>SYDTVMDKYWLSQYVIARETYDWYTLQKDYETVGMLSSPSEGQSYASQFQGDKALDKQYGSNVRTSVTIVSIVPNGKGIGTVRFAKTTKRTNETGDGETTHWIA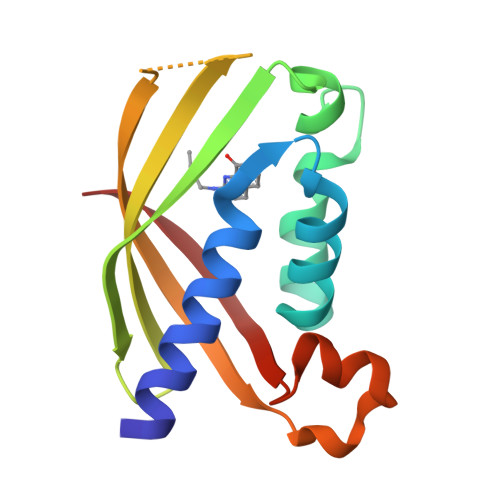TIGYQYVNPSLMSESARLTNPLGFNVTSYRVDPE[5x]~{N}-[3-[[5-cyclopropyl-2-[(2-methyl-3,4-dihydro-1~{H}-isoquinolin-6-yl)amino]pyrimidin-4-yl]amino]propyl]cyclobutanecarboxamide 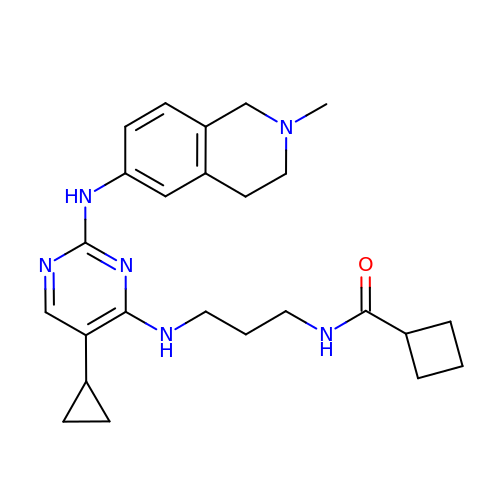| C25 H34 N6 O | KKISLZKMBSCLSS-UHFFFAOYSA-N>GPHMDYKFWYTQPVPKINDEFNESVNEPFISDNKVEDVRKDEYKLPPGYSWYVCDVKDEKDRSEIYTLLTDNYVEDDDNIFRFNYSAEFLLWALTSPNYLKTWHIGVKYDASNKLIGFISAIPTDICIHKRTIKMAEVNFLCVHKTLRSKRLAPVLIKEITRRINLENIWQAIYTAGVYLPKPVSDARYYHRSINVKKLIEIGFSSLNSRLTMSRAIKLYRVEDTLNIKNMRLMKKKDVEGVHKLLGSYLEQFNLYAVFTKEEIAH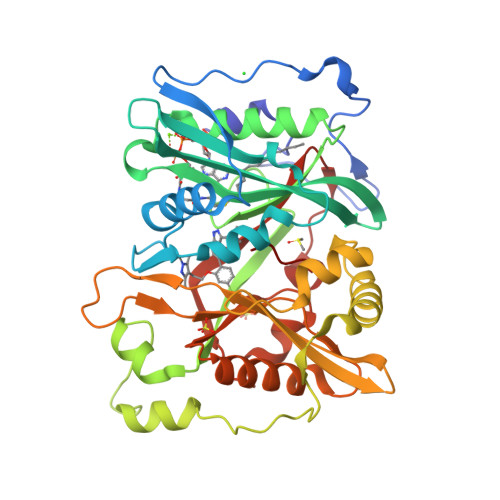WFLPIENVIYTYVNEENGKIKDMISFYSLPSQILGNDKYSTLNAAYSFYNVTTTATFKQLMQDAILLAKRNNFDVFNALEVMQNKSVFEDLKFGEGDGSLKYYLYNWKCASFAPAHVGIVLL[3x]>[2x]GRSRLLEDFRNNRYPNLQLREIAGHIMEFSQDQHGSRFIQLKLERATPAERQLVFNEILQAAYQLMVDVFGNYVIQKFFEFGSLEQKLALAERIRGHVLSLALQMYGCRVIQKALEFIPSDQQNEM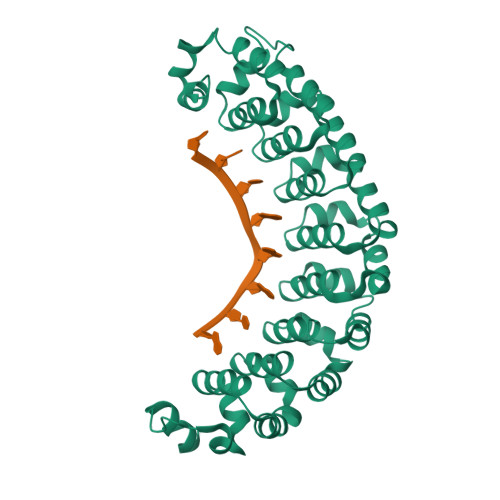VRELDGHVLKCVKDQNGNHVVQKCIECVQPQSLQFIIDAFKGQVFALSTHPYGCRVIQRILEHCLPDQTLPILEELHQHTEQLVQDQYGNYVIQHVLEHGRPEDKSKIVAEIRGNVLVLSQHKFASNVVEKCVTHASRTERAVLIDEVCTMNDGPHSALYTMMKDQYANYVVQKMIDVAEPGQRKIVMHKIRPHIATLRKYTYGKHILAKLEKYYMKNGVDLG>[2x]AEPLDVVATFSIIGDFAAKVGGDRIRLNVLVGPDSDTHVYEPRPADAIALAGADVVLTNGLEFEGFLTRLIAASGTDAAVATLTDGVETMEEPGGGHYHYIDGKAVFHAGAHDPHAWQAVPNAKVYVQNIAAAFCAADAEGCAAYQAN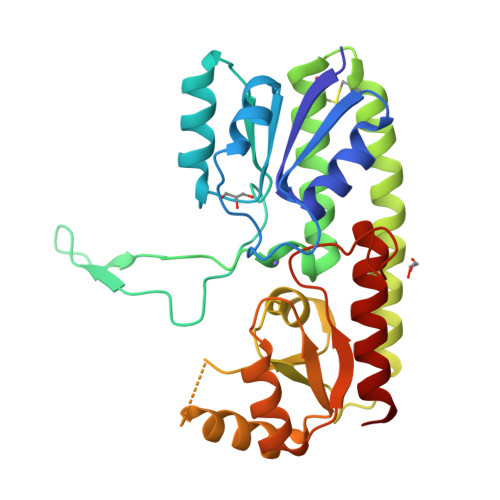AARYIGELDALDTEIRAAIAALPQDRRTVVVAHNAFRYFEAAYGVHFLSPQGVSTESEAAAADVAGLIREIRARNASAIFAENISDTRLLEQIAREAGLPLAGTLYSDALSGPDGPASNYIAMMRHNAGAIAAALAAR>MSRLYKDICSLRTLYGAWRKVRSSAFLSSSDEIRREAEEFESRLPDSLIEIQHALSKQIFIFLQQTGVAQKKPGGKSRPLVLAPIPNRVVQRALLDVLQRRVRLVKRVLGTPTSYGGIPDKRVAMAIADAREAMRTGARFHIRSDIPAFF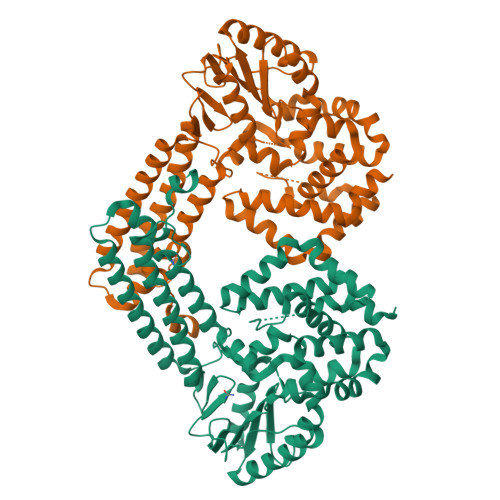TKINKDRVLELLRPHLNCEATLKLFEEAIRTDLANIDDLRRKGLDEIFPIGIEGVAQGSPLSPLLANIYLADFDLAMNSNGITCLRYIDDFLLLGASLSDVDKAFNRALKELGKIGLEAYDPRTDKTKASRGATEIGFDFLGCNVSPGLIQPSEATRRRFRAKLDAEFVAASHALRYNAQYQDGDGKYSYSSALYRIDKIILGWGKAFTFCNGSQCMIALDDFISNKLAQLEAEKIAILANSDSTVRRRVLGVRLLIDIQN[2x]> MKKIALIIGSMIAGGIISAAGFTWVAKAEPPAEKTSTAERKILFWYDPMYPNTRFDKPGKSPFMDMDLVPKYADEESSASGVRIDPTQTQNLGVKTATVTRGPLTFAQSFPANVSYNEYQYAIVQARAAGFIDKVYPLTVGDKVQKGTPLLDLTIPDWVEAQSEYLLLRETGGTATQTEGILERLRLAGMPEADIRRLIATQKIQTRFTLKAPIDGVITAFDLRAGMNIAKDNVVAKIQGMDPVWVTAAIPESIAWLVKDASQFTLTVPARPDKTLTIRKWTLLPG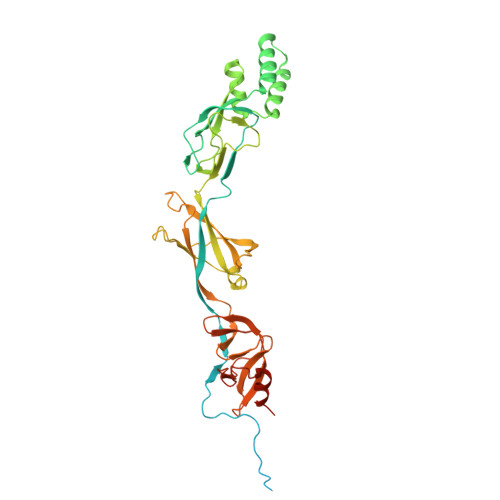VDAATRTLQLRLEVDNADEALKPGMNAWLQLNTASEPMLLIPSQALIDTGSEQRVITVDADGRFVPKRVAVFQASQGVTALRSGLAEGEKVVSSGLFLIDSEANISGALERMRSESATHAHHHHHHH>MTATVLLEVPFSARGDRIPDAVAELRTREPIRKVRTITGAEAWLVSSYALCTQVLEDRRFSMKETAAAGAPRLNALTVPPEVVNNMGNIADAGLRKAVMKAITPKAPGLEQFLRDTANSLLDNLITEGAPADLRNDFADPLATALHCKVLGIPQEDGPKLFRSLSIAFMSSADPIPAAKINWDRDIEYMAGILENPNITTGLMGELSRLRKDPAYSHVSDELFATIGVTFFGAGVISTGSFLTTALISLIQRPQLRNLLHEKPELIPAGVEELLRINLSFADGLPRLATADIQVGDVLVRKGELVLVLLEGANFDPEHFPNPGSIELDRPNPT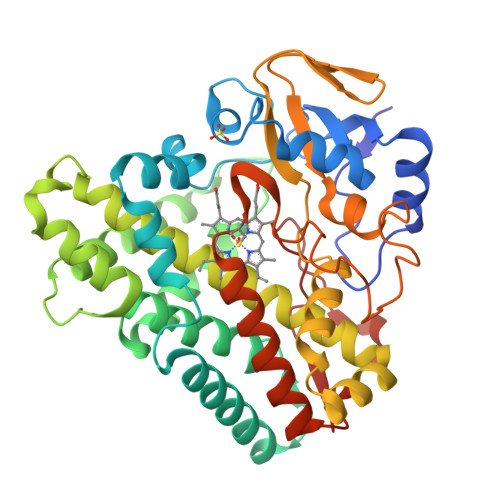SHLAFGRGQHFCPGSALGRRHAQIGIEALLKKMPGVDLAVPIDQLVWRTRFQRRIPERLPVLW[6x]> TEFLKPRLVDIEQVSSTHAKVTLEPLERGFGHTLGNALRRIL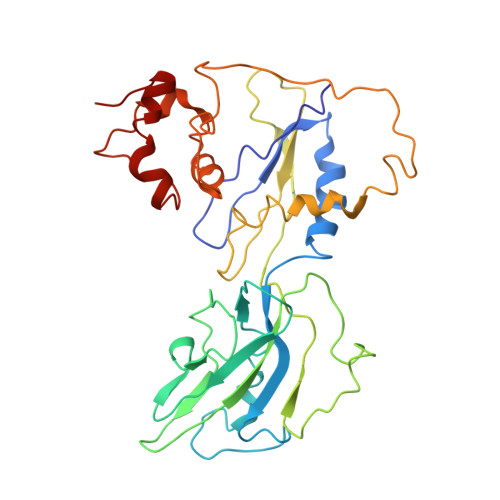LSSMPGCAVTEVEIDGVLHEYSTKEGVQEDILEILLNLKGLAVRVQGKDEVILTLNKSGIGPVTAADITHDGDVEIVKPQHVICHLTDENASISMRIKVQRGRGYVPASTRIHSEEDERPIGRLLVDACYSPVERIAYNVEAARVEQRTDLDKLVIEMETNGTIDPEEAIRRAATILAEQLEAFVDLRDVRQPEVKEEKPEFDPILLLPVDDLELTVRSANCLKAEAIHYIGDLVQRTEVELLKTPNLGKKSLTEIKDVLASRGLSLG4-(aminomethyl)-~{N}-[(1~{S})-1-[4-(3-oxidanyl-1~{H}-indazol-5-yl)pyridin-2-yl]-2-phenyl-ethyl]cyclohexane-1-carboxamide | C28 H31 N5 O2 | 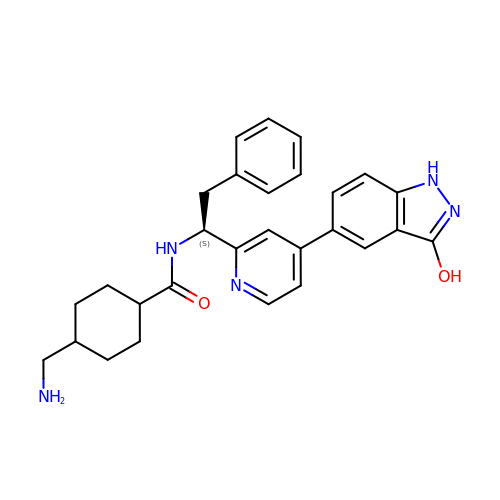OTOUCEKJIQXXLM-DYLHXGEVSA-N>PPHGELQYLGQI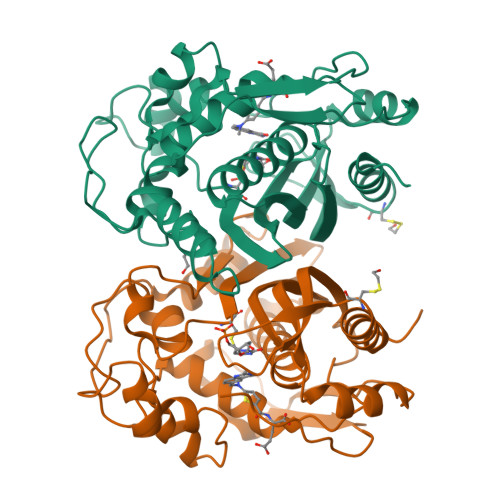QHILRCGVRKDDRTGTGTLSVFGMQARYSLRDEFPLLTTKRVFWKGVLEELLWFIKGSTNAKELSSKGVKIWDANGSRDFLDSLGFSTREEGDLGPVYGFQWRHFGAEYRDMESDYSGQGVDQLQRVIDTIKTNPDDRRIIMCAWNPRDLPLMALPPCHALCQFYVVNSELSCQLYQRSGDMGLGVPFNIASYALLTYMIAHITGLKPGDFIHTLGDAHIYLNHIEPLKIQLQREPRPFPKLRILRKVEKIDDFKAEDFQIEGYNPHPTIKMEMAV[4x]>MAKKVNWYVSCSPRSPEKIQPELKVLANFEGSYWKGVKGYKAQEAFAKELAALPQFLGTTYKKEAAFSTRDRVAPMKTYGFVFVDEEGYLRITEAGKMLANNRRPKDVFLKQLVKWQYPSFQHKGKEYPEEEWSINPLVFVLSLLKKVGGLSKLDIAMFCLTATNNNQVDEIAEEIMQFRNEREKIKGQNKKLEFTENYFFKRFEKIYGNVGKIREGKSDSSHKSKIETKMRNARDVADATTRYFRYTGLFVARGNQLVLNPEKSDLIDEIISSSKVVKNYTRVEEFHEYYGNPSLPQFSFETKEQLLDLAHRIRDENTRLAEQLVEHFPNVKVEIQVLEDIYNSLNKKVDVETLKDVIYHAKELQLELKKKKLQADFNDPRQLEEVIDLLEVYHEKKNVIEEKIKARFIANKNTVFAWLTWNGFIILGNALEYKNNFVIDEELQPVTHAAGNQPDMEIIYEDFIVLGEVTTSKGATQFKMESEPVTRHYLNKKKELEKQGVEKELYCLFIAPEINKNTFEEFMKYNIVQN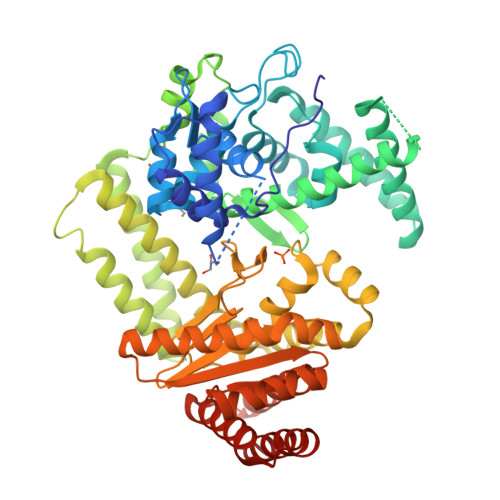TRIIPLSLKQFNMLLMVQKKLIEKGRRLSSYDIKNLMVSLYRTTIECERKYTQIKAGLEETLNNWVVDKEVRF[2x]>MTVGNDDNLDKEIGQLLMCGFDGLEPTPGIIDLIENHNLGSIILFSRNIATPKQVQKLTHSLQQIARNAGHKRPLFIAVDQENGVVRRLGDSGTYLPGNMALGALGSSTAARNVAMAISKELLTLGMNWNLAPVLDVNNNPLNPVIGVRSYGQDPELVARMGLAQVEGYQRGKVATSIKHFPGHGDTATDSHLDVPVINKTLEELDKTELVPFKKALEAGGIACPTSVMVGHMLLPHFNKDVVSSIAPEIVRDLLRRRFGYKGVIITDCLEMDAVKETVGTPKGALMALQAGNDMAMISHTLAFQKDAFKVLYSALQEGQLDKDEIRQSLQRVAQLKDQFLNWDDVLQQADLKTMGSEAHATLSKELYDRVPTVVTNRKNTLPIRPAQTDKILFLAAHVPQTLAVDSEKEPFNSFHASLLKRHTNLEYIIYNEETPDLSQKIQEADWVIIGTANANLYPFQVRMVQQAQKLAKRLVVAAVMNPYDQMCFPQVDTYLVTYEYTPPAHEAAVRLIFGEIETRSRLPISIPNVDDAIAPATFIVDDYRNDDDLDHVTAMWDDIFGKDWPLRKDKINLGLQRAKLQKHKVARDSQGKIVGFVATQIVVVDNKKHGQLMLLMVSPSYQGKGVGTLLHDAALEHFREQGADCIKLGSTYPRFFPGVPDDDAQSRKAQAFFSKKGWRMDDNLVHDLIGDLQDYKVPDKIQARMLKEKIWFGRIKPSETWELYAFQQRNFPHWLSTYQHHVELGDYQDLIVARQDDENGRVIASLILNTTHVSHEYRSDLIWTDDKLFGERSGGMACVGVAQEERGRGIGIGIVAHANWLLKQRGVTKSYVDWVELLDFYSRVGYKTWRSYRLGHF[2x]

The full-length β-N-acetylglucosaminidase (RmNag) from Rhizomucor miehei belongs to glycoside hydrolase (GH) family 3 in the CAZy classification of carbohydrate-active enzymes and the characterisation of which has been reported in our previous study16. RmNag is a 858-amino-acid protein with multiple distinctive structural domains and the β-N-acetylglucosaminidase activity lies in the N-terminal region. In the present study, the crystal structure of full-length RmNag has been resolved to 2.8 Å resolution to find that a unique GCN5-related N-acetyltransferase region exists in the C-terminal region of RmNag, which displays glucosamine N-acetyltransferase activity in vitro. The crystal structure of full-length RmNag reveals two distinct functional regions: a β-N-acetylglucosaminidase N-terminal region (NTR, domains A and B, residues 26–529), and a N-acetyltransferase C-terminal region (CTR, domains C and D, residues 537–858).

The monoclinic space group of RmNag was P4212 with two monomers in the asymmetric unit. However, the β-N-acetylglucosaminidase region (NTR) and the N-acetyltransferase region (CTR) are monomeric and dimeric in solution, respectively, indicating that full-length RmNag dimerizes via the interactions owing to its CTR. The N-terminal domain (domain A, residues 26–371) reveals a characteristic (β/α)8 TIM barrel, which is typical for catalytic domains of GH family 3 members. The C-terminal domain (domain B, residues 372–529) displays a 3α/6β/3α sandwich-like fold, in which a six-stranded β-sheet is sandwiched by two layers of three helices each. In the structure of RmNag, a non-canonical His192/Asp190 dyad able to function as the catalytic acid/base is present on a flexible loop which is 6.3 Å apart from the conserved aspartate nucleophile (Asp268). The N-acetyltransferase C-terminal region (CTR) of RmNag contained two structurally conserved GNAT-fold domains (C and D). A co-purified AcCoA molecule was found in the N-terminal of CTR (domain C, Ala537–Leu693). However, this AcCoA molecule and the domain C are unlikely to be directly involved in acetyl transfer, mainly because there are no residues nearby the acetyl group that can be possibly involved in general acid/base catalysis. Consequently, the acetyl transfer activity must be located within the C-terminal of CTR (domain D, Ile711–Phe858). Most important, the conserved tyrosine (Y842 in RmNag) which has been predicted to act as the general acid to protonate the leaving thiolate anion nearly overlapped with the one of the HsGNA1–CoA–GlcNAc-6P complex and it is therefore within hydrogen bond distance from the sulphur atom of a bound CoA.> MNDQIKIRKATKEDWEKIYQLYNSLSDEDLYLRFFHLYRITEEDAKKIAS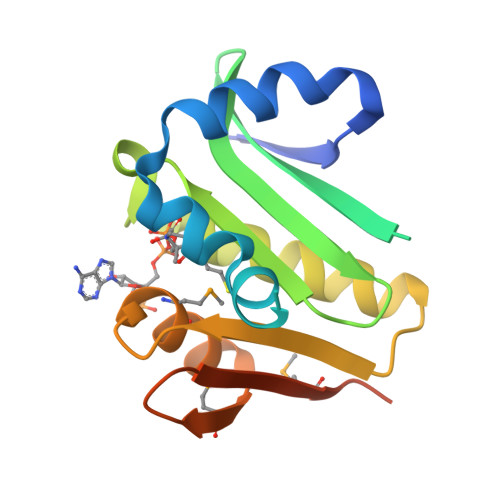NEDHVTFLAEVDGKVVGEASLHKDGEFSLVVHRNYRTLGIGTLLVKTLIEEAKKSGLSTVKFYTLPENTPMIKIGRKLGFKMRFYEDEVYGEMRLTERELNVNLATFSAP> SDRVLQLKLGNSAIVTQEAANYCCAYGEWPNYLPDHEAVAIDKPTQPETATDRFYTLKSVKWETGSTGWWWKLPDALNNIGMFGQNVQHHYLYRSGFLIHVQCNATKFHQGALLVVAIPEHQRGAHNTNTSPGFDDIMKGEEGGTFNHPYVLDDG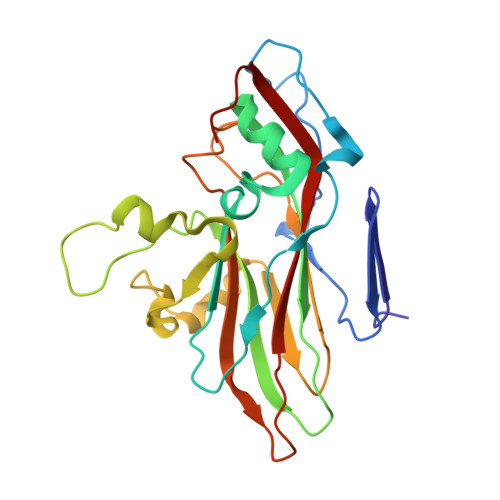TSLACATIFPHQWINLRTNNSATIVLPWMNAAPMDFPLRHNQWTLAIIPVVPLGTRTTSSMVPITVSIAPMCCEFNGLRHAIT> SDTGRPFVEMYSEI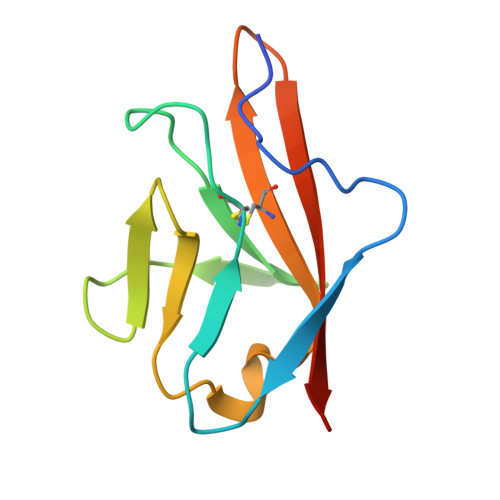PEIIHMTEGRELVIPCRVTSPNITVTLKKFPLDTLIPDGKRIIWDSRKGFIISNATYKEIGLLTCEATVNGHLYKTNYLTHRQTNTI>[2x]LSTSLSALPAAARDFVEEAVRLCRPREVLLCDGSEEEGKELLRGLQDDGVLHPLPKYDNCWLARTDPRDVARVES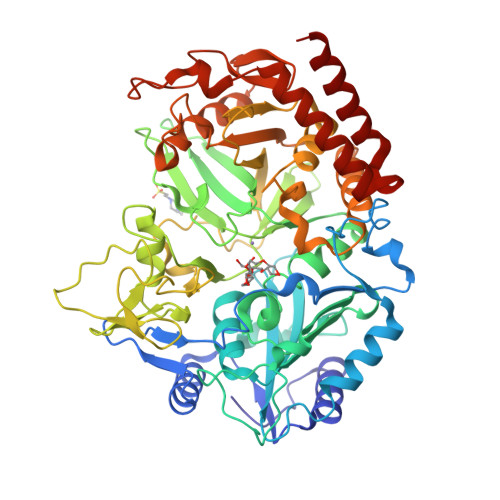KTVLVTPEQSDAVPPPPPSGGPPQLGNWMSPNAFQAAVQERFPGCMAGRPLYVIPFSMGPPTSPLAKLGVQVTDSPYVVLSMRIMTRVGPAVLQRLDDDFVRCLHSVGRPLPLTEPLVSSWPCDPSRVLVAHIPSERRIVSFGSGYGGNSLLGKKCFALRIASRMAQQQGWLAEHMLILGVTSPSGEKRYMAAAFPSACGKTNLAMMTPSLPGWRIHCVGDDIAWMKFDDEGRLRAINPERGFFGVAPGTSSRTNPNAMATIARNTIFTNVGLRSDGGVYWDGLDEPTEPGVTYTSWLGKPWKHGDPEPCAHPNSRFCAPADQCPIMDPRWDDPEGVPIDAIIFGGRRPRGVPLVVEAFGWRHGVFMGSAMRSEATAAAEHKGGRLMHDPFAMRPFFGYNAGRYLEHWLSTGLRSNARLPRLFHVNWFLRDNEGRFVWPGFGHNARVLAWIFGRIQGRDTARPTPIGWVPKEGDLDLGGLPGVDYSQLFPMEKGFWEEECRQLREYYGENFGADLPRDVMAELEGLEERVRKM> ESAPDPVLDTEGKQLRSGVDYYILPVIRGRGGGLTLASTGNENCPLDVVQEQHEVSNGLPLTFTPVNPKKGVIRVSTDHNIKFSASTICVQSTLWKLEYDESSGQRFVTTGGVEGNPGRETLDNWFKIEKYEDDYKLVFCPTVCDFCKPVCGDIGIYIQ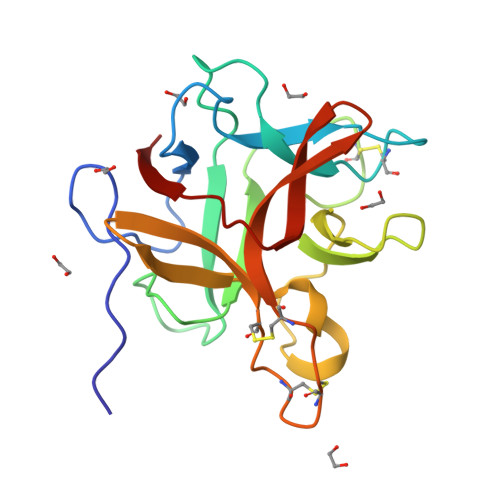NGYRRLALSDVPFKVMFKKA> SSQSSSP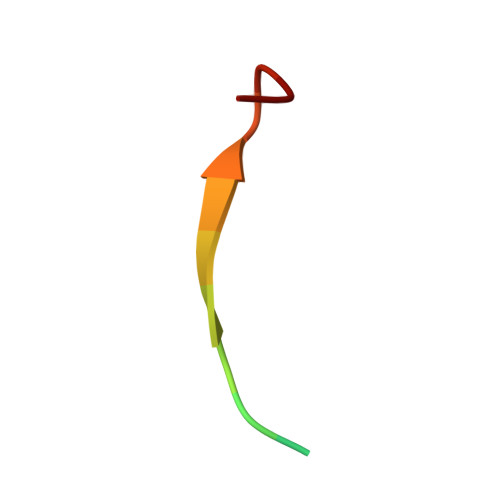TEMDENES> TNEY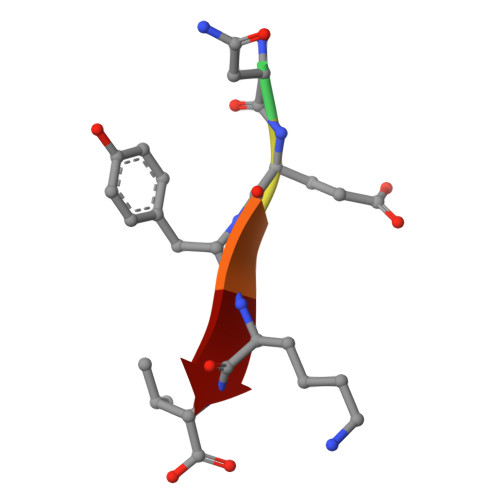KV> RDQAGITGTWYNQLGS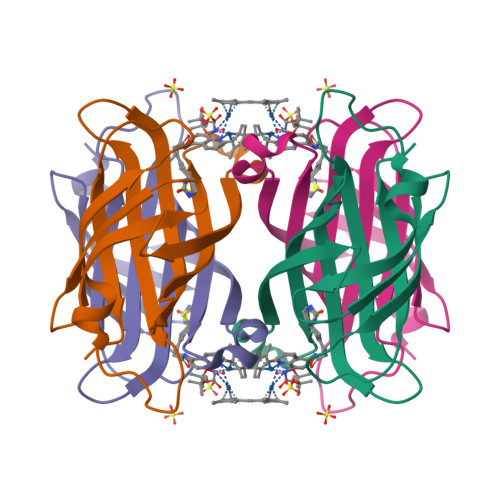TFIVTAGADGALTGTYESAVGNAESRYVLTGRYDSAPATDGSGTALGWTVAWKNNYRNAHSATTWSGQYVGGAEARINTQWLLTSGTTEANAWKSTLVGHDTFTKVK> MKRGFARPTPEKPPVIKPENIVLSTPLSIPPPEGKPWWLIVVGVVVVGLLGGMVAMVFASGSHVFGGIGSIFPLFMMVGIMMMMFRGMGGGQQQMSRPKLDAMRAQFMLMLDMLRETAQESADSMDANYRWFHPAPNTLAAAVGSPRMWERKPDGKDLNFGVVRVGVGMTRPEVTWGEPQNMPTDIELEPVTGKALQEFGRYQSVVYNLPKMVSLLVEPWYALVGEREQVLGLMRAIICQLAFSHGPDHVQMIVVSSDLDQWDWVKWLPHFGDSRRHDAAGNARMVYTSVREFAAEQAELFAGRGSFTPRHASSSAQTPTPHTVIIADVDDPQWEYVISAEGVDGVTFFDLTGSSMWTDIPERKLQFDKTGVIEALPRDRDTWMVI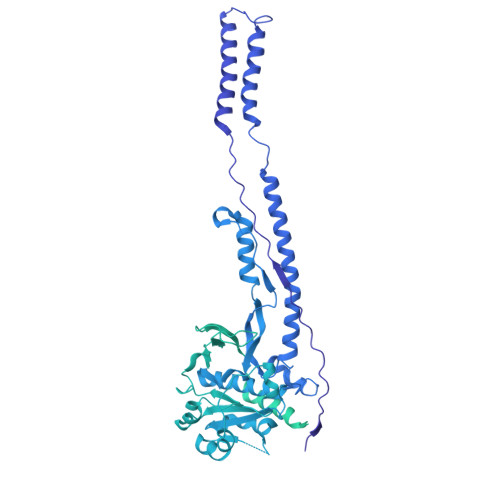DDKAWFFALTDQVSIAEAEEFAQKLAQWRLAEAYEEIGQRVAHIGARDILSYYGIDDPGNIDFDSLWASRTDTMGRSRLRAPFGNRSDNGELLFLDMKSLDEGGDGPHGVMSGTTGSGKSTLVRTVIESLMLSHPPEELQFVLADLKGGSAVKPFAGVPHVSRIITDLEEDQALMERFLDALWGEIARRKAICDSAGVDDAKEYNSVRARMRARGQDMAPLPMLVVVIDEFYEWFRIMPTAVDVLDSIGRQGRAYWIHLMMASQTIESRAEKLMENMGYRLVLKARTAGAAQAAGVPNAVNLPAQAGLGYFRKSLEDIIRFQAEFLWRDYFQPGVSIDGEEAPALVHSIDYIRPQLFTNSFTPLEVSVGGPDIEPVVAQPNGEVLESDDIEGGEDEDEEGVRTPKVGTVIIDQLRKIKFEPYRLWQPPLTQPVAIDDLVNRFLGRPWHKEYGSACNLVFPIGIIDRPYKHDQPPWTVDTSGPGANVLILGAGGSGKTTALQTLICSAALTHTPQQVQFYCLAYSSTALTTVSRIPHVGEVAGPTDPYGVRRTVAELLALVRERKRSFLECGIASMEMFRRRKFGGEAGPVPDDGFGDVYLVIDNYRALAEENEVLIEQVNVIINQGPSFGVHVVVTADRESELRPPVRSGFGSRIELRLAAVEDAKLVRSRFAKDVPVKPGRGMVAVNYVRLDSDPQAGLHTLVARPALGSTPDNVFECDSVVAAVSRLTSAQAPPVRRLPARFGVEQVRELASRDTRQGVGAGGIAWAISELDLAPVYLNFAENSHLMVTGRRECGRTTTLATIMSEIGRLYAPGASSAPPPAPGRPSAQVWLVDPRRQLLTALGSDYVERFAYNLDGVVAMMGELAAALAGREPPPGLSAEELLSRSWWSGPEIFLIVDDIQQLPPGFDSPLHKAVPFVNRAADVGLHVIVTRTFGGWSSAGSDPMLRALHQANAPLLVMDADPDEGFIRGKMKGGPLPRGRGLLMAEDTGVFVQVAATEVRR>PEDELKRVEKLVKEAEALLIVAKIKGSKRDLEKALRTAEEAAREAVKVLVQALLEGDPEVALRAVELVVRVAELLLRIAKESGSREALLRALIVAEEAAKLAKMVLELAEKQGDPEVALRAVELVVRVAELLLRIAKESGSEEALERALRVAEEAARLAKRVLELAEEQGDPLV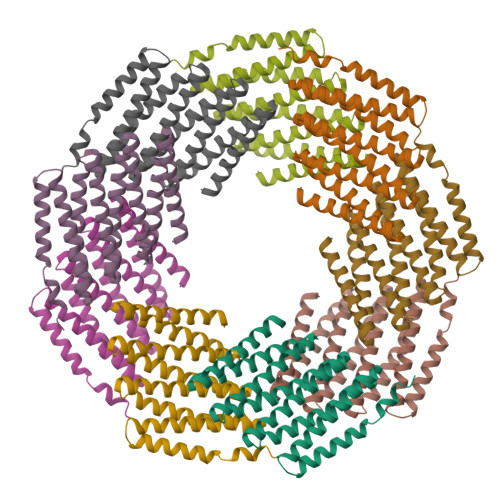AKMAVELVKRVAELLERIARESGSEEAKERAERVREEARELQERVKELRER[9x]> MARAAFLFKTVGFGGLQNVPINDELSSHLLRAGNSPWQLTQFLDWISLGRGLATSA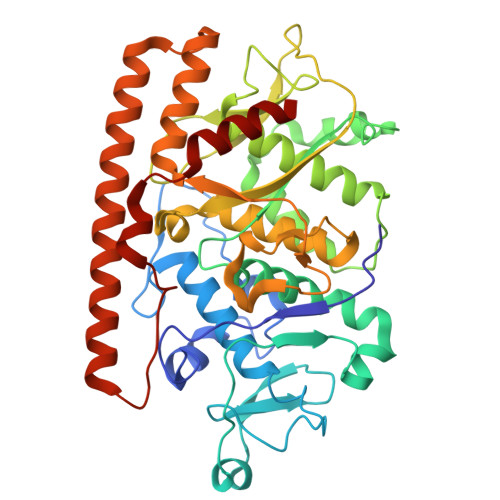LVPTAGSRYYQMSCLLSGTLQIPFRPNHRWGDIRFLRLVWSAPTLDGLVVAPPQVLAQPALQAQADRVYDCDDYPFLARDPRFKHRVYQQLSAVTLLNLTGFGPISYVRVDEDMWSGDVNQLLMNYFGHTFAEIAYTLCQASANRPWEYDGTYARMTQIVLSLFWLSYVGVIHQQNTYRTFYFQCNRRGDAAEVWILSCSLNHSAQIRPGNRSLFVMPTSPDWNMDVNLILSSTLTGCLCSGSQLPLIDNNSVPAVSRNIHGWTGRAGNQLHGFQVRRMVTEFCDRLRRDGVMTQAQQNQVEALADQTQQFKRDKLETWAREDDQYNQAHPNSTMFRTKPFTNAQWGRGNTGATSAAIAALI>[2x]MSSEANPPVLEPFTVTVVDRNVKHQVEGEPEEEGHPDHEVQGVMFATNVKYIFEDDQELLPEQEDPAIENVVIIEADESLRVTQVEMISDQFKQVGYEVRDGNEVCIDAMSRFETPRQLGNLPLEKLVQLYKLQNDQLHSLFNTLAGQFYLNAHHHHHH;>[2x]MNEAVIEKLLENSRKFLTGAKLICQESNDHLTTTKLRIREWQKFQSKLHFVLDCIQQQTKFLSEILLREGIGRNLIEEEWSQTVLVRLV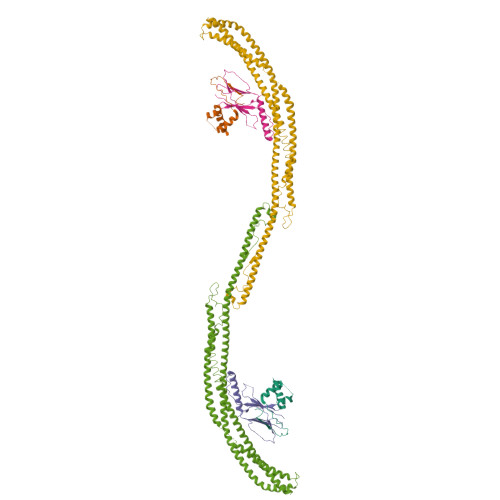NDMKFWQNEITKMMNKLDNITNEIDQQHNSKLGDFISRDSSHILDSKLNEIPTIRKQVENITRQYQTMLAKVQSQLVESRMKGLRDEFSSKFGDQCRENLKLNEEFTNEADQLEQELADFLKSFTDHFDKCSALSSRSVSPEDAQNLFEIVERDDKDLAAINSLLQDAAIDVASFVRKVNMLLDERDADKAKMQATLSKLLTELRKHEEYISVFEGISALIQKFKASCLEDIRQTRNLLDFYANFERSYHNLLKEVKRRKETAAKLSQILKSCETQLEQINTADLRERQMFLLENGNYLPETIWPDEIGSLSPLYTLNYEVRKV>NYSNEFGLMQPIQEFKAFIESDPVVHQEFIDMFEGIQDSPRNYQELCNMFNDIFRKAPVYGDLGPPVYMIMAKLMNTRAGFSAFTRQRLNLHFKKLFDTWGLFLSSKDSRNVLVADQFDDRHCGWLNERALSAMVKHYNGRAFDEVFLCDKNAPYYGFNSYDDFFNRRFRNRDIDRPVVGGVNNTTLISAACESLSYNVSYDVQSLDTLVFKGETYSLKHLLNNDPFTPQFEHGSILQGFLNVTAYHRWHAPVNGTIVKIINVPGTYFAQAPSTIGDPIPDNDYDPPPYLKSLVYFSNIAARQIMFIEADNKEIGLIFLVFIGMTEISTCEATVSEGQHVNRGDDLGMFHFGG[2x];>XSFALG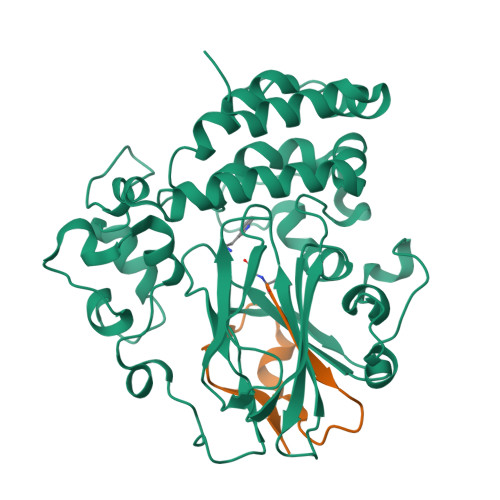LRKDCRAEIVEKFTEPGTVIRINEVVAALKA[2x]>[2x]MAREFSLEKTRNIGIMAHIDAGKTTTTERILYYTGRIHKIGETHEGASQMDWMEQEQDRGITITSAATTAAWEGHRVNIIDTPGHVDLTVEVERSLRVLDGAVTVLDA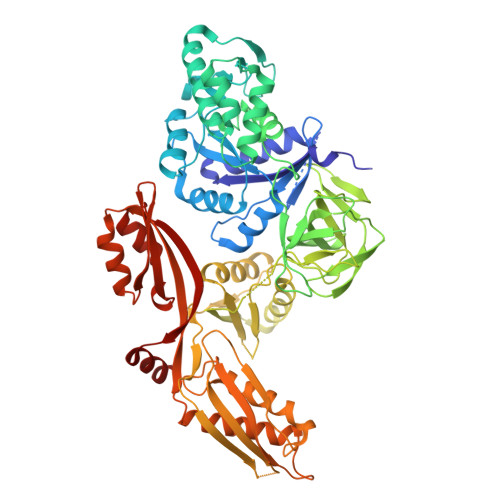QSGVEPQTETVWRQATTYGVPRIVFVNKMDKLGANFEYSVSTLHDRLQANAAPIQLPIGAEDEFEAIIDLVEMKCFKYTNDLGTEIEEIEIPEDHLDRAEEARASLIEAVAETSDELMEKYLGDEEISVSELKEAIRQATTNVEFYPVLCGTAFKNKGVQLMLDAVIDYLPSPLDVKPIIGHRASNPEEEVIAKADDSAEFAALAFKVMTDPYVGKLTFFRVYSGTMTSGSYVKNSTKGKRERVGRLLQMHANSRQEIDTVYSGDIAAAVGLKDTGTGDTLCGEKNDIILESMEFPEPVIHLSVEPKSKADQDKMTQALVKLQEEDPTFHAHTDEETGQVIIGGMGELHLDILVDRMKKEFNVECNVGAPMVSYRETFKSSAQVQGKFSRQSGGRGQYGDVHIEFTPNETGAGFEFENAIVGGVVPREYIPSVEAGLKDAMENGVLAGYPLIDVKAKLYDGSYHDVDSSEMAFKIAASLALKEAAKKCDPVILEPMMKVTIEMPEEYMGDIMGDVTSRRGRVDGMEPRGNAQVVNAYVPLSEMFGYATSLRSNTQGRGTYTMYFDHYAEVPKSIAEDIIKKNKGE>GSPNSMQEKDASSQGFLPHFQHFATQAIHVGQDPEQWTSRAVVPPISLSTTFKQGAPGQHSGFEYSRSGNPTRNCLEKAVAALDGAKYCLAFASGLAATVTITHLLKAGDQIICMDDVYGGTNRYFRQVASEFGLKISFVDCSKIKLLEAAITPETKLVWIETPTNPTQKVIDIEGCAHIVHKHGDIILVVDNTFMSPYFQRPLALGADISMYSATKYMNGHSDVVMGLVSVNCESLHNRLRFLQNSLGAVPSPIDCYLCNRGLKTLHVRMEKHFKNGMAVAQFLESNPWVEKVIYPGLPSHPQHELVKRQCTGCTGMVTFYIKGTLQHAEIFLKNLKLFTLAESLGGFESLAELPAIMTHASVLKNDRDVLGISDTLIRLSVGL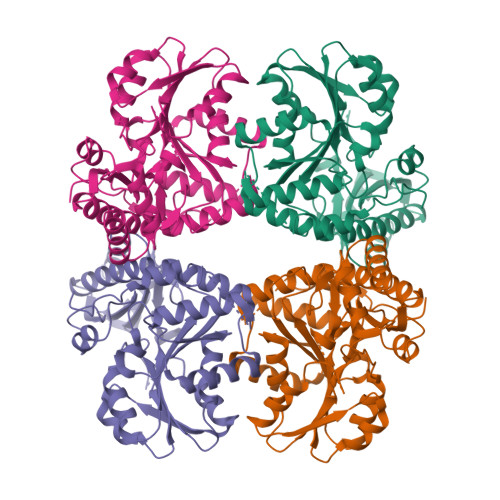EDEEDLLEDLDQALKAAHPPSGSHS[4x]> SQKSWIESTLTKRECVYIIPSSKDPHRCLPGCQICQQLVRCFCGRLVKQHACFTASLAMKYSDVKLGEHFNQAIEEWSVEKHTEQSPTDAYGVINFQGGSHSYRAKYVRLSYDTKPEIILQLLLKEWQMELPKLVISVHGGMQKFELHPRIKQLLGKGLIKAAVTTGAWILTGGVNTGVAKHVGDALKEHASRSSRKICTIGIAPWGVIENRNDLVGRDVVAPYQTLLNPLSKLNVLNNLHSHFILVDDGTVGKYGAEVRLRRELEKTINQQRIHARIGQGVPVVALIFEGGPNVILTVLEYLQESPPVPVVVCEGTGRAADLLAYIHKQTEEGGNLPDAAEPDIISTIKKTFNFGQSEAVHLFQTMMECMKKKELITVFHIGSEDHQDIDVAILTALLKGTNASAFDQLILTLAWDRVDIAKNHVFVYGQQWLVGSLEQAMLDALVMDRVSFVKLLIENGVSMHKFLTIPRLEELYNTKQGPTNPMLFHLIRDVKQGNLPPGYKITLIDIGLVIEYLMGGTYRCTYTRKRFRLIYNSLGGNNRRSGRNTSSSTPQLRKSHETFGNRADKKEKMRHNHFIKTAQPYRPKMDASMEEGKKKRTKDEIVDIDDPETKRFPYPLNELLIWACLMKRQVMARFLWQHGEESMAKALVACKIYRSMAYEAKQSDLVDDTSEELKQYSNDFGQLAVELLEQSFRQDETMAMKLLTYELKNWSNSTCLKLAVSSRLRPFVAHTCTQMLLSDMWMGRLNMRKNSWYKVILSILVPPAILMLEYKTKAEMSHIPQSQDAHQMTMEDSENNFHNITEEIPMEVFKEVKILDSSDGKNEMEIHIKSKKLPITRKFYAFYHAPIVKFWFNTLAYLGFLMLYTFVVLVKMEQLPSVQEWIVIAYIFTYAIEKVREVFMSEAGKISQKIKVWFSDYFNVSDTIAIISFFVGFGLRFGAKWNYINAYDNHVFVAGRLIYCLNIIFWYVRLLDFLAVNQQAGPYVMMIGKMVANMFYIVVIMALVLLSFGVPRKAILYPHEEPSWSLAKDIVFHPYWMIFGEVYAYEIDVCANDSTLPTICGPGTWLTPFLQAVYLFVQYIIMVNLLIAFFNNVYLQVKAISNI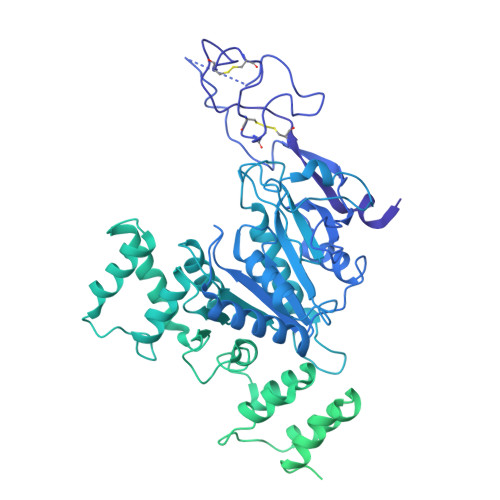VWKYQRYHFIMAYHEKPVLPPPLIILSHIVSLFCCVCKRRKKDKTSDGPKLFLTEEDQKKLHDFEEQCVEMYFDEKDDKFNSGSEERIRVTFERVEQMSIQIKEVGDRVNYIKRSLQSLDSQIGHLQDLSALTVDTLKTLTAQKASEASKVHNEITRELSISKHLAQNLID> IFNGRPAQKGTTPWIAMLSHLNGQPFCGGSLLGSSWIVTAAHCLHQSLDPKDPTLRDSDLLSPSDFKIILGKHWRLRSDENEQHLGVKHTTLHPQYDPNTFENDVALVELLESPVLNAFVMPICLPEGPQQEGAMVIVSGWGKQFLQRFPETLMEIEIPIVDHST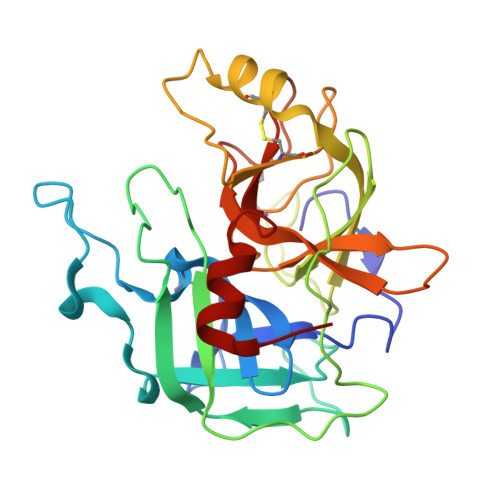CQKAYAPLKKKVTRDMICAGEKEGGKDACAGDSGGPMVTLNRERGQWYLVGTVSWGDDCGKKDRYGVYSYIHHNKDWIQRVTGVRN> MSSVTWAPGNYPSTRRSDHVDTYQSASKGEVPVPDPYQW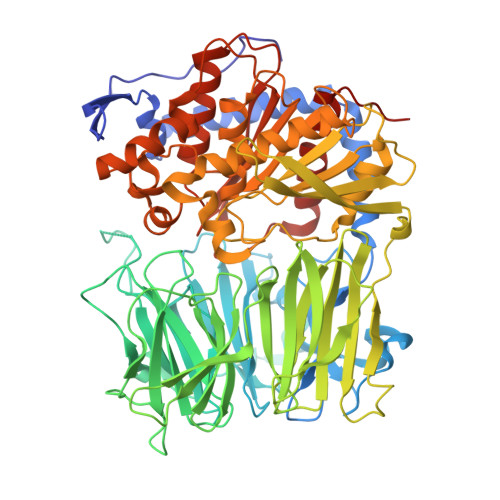LEESTDEVDKWTTAQADLAQSYLDQNADIQKLAEKFRASRNYAKFSAPTLLDDGHWYWFYNRGLQSQSVLYRSKEPALPDFSKGDDNVGDVFFDPNVLAADGSAGMVLCKFSPDGKFFAYAVSHLGGDYSTIYVRSTSSPLSQASVAQGVDGRLSDEVKWFKFSTIIWTKDSKGFLYQRYPARERHEGTRSDRNAMMCYHKVGTTQEEDIIVYQDNEHPEWIYGADTSEDGKYLYLYQFKDTSKKNLLWVAELDEDGVKSGIHWRKVVNEYAADYNIITNHGSLVYIKTNLNAPQYKVITIDLSKDEPEIRDFIPEEKDAKLAQVNCANEEYFVAIYKRNVKDEIYLYSKAGVQLTRLAPDFVGAASIANRQKQTHFFLTLSGFNTPGTIARYDFTAPETQRFSILRTTKVNELDPDDFESTQVWYESKDGTKIPMFIVRHKSTKFDGTAAAIQYGYGGFATSADPFFSPIILTFLQTYGAIFAVPSIRGGGEFGEEWHKGGRRETKVNTFDDFIAAAQFLVKNKYAAPGKVAINGASNGGLLVMGSIVRAPEGTFGAAVPEGGVADLLKFHKFTGGQAWISEYGNPSIPEEFDYIYPLSPVHNVRTDKVMPATLITVNIGAGRVVPMHSFKFIATLQHNVPQNPHPLLIKIDKSWLGHGMGKPTDKNVKDAADKWGFIARALGLELKTVE> GSHHHHHHSIETDRVSKEFIEFLKTFHKTGQEIYKQTKLFLEGMHYKRDLSIEEQSECAQDFYHNVAERMQTRGKVPPERVEKIMDQIEKYIMTRLYKYVFCPETTDDEKKDLAIQKRIRALRWVTPQMLCVPVNEDIPEVSDMVVKAITDIIEMDSKRVPRDKLACITKCSKHIFNAIKITKNEPASADDFLPTLIYIVLKGNPPRLQSNIQYITRFCNPSRLMTGEDGYYFTNLCCAVAFIEKLDAQSLNLSQEDFDRYMSGQTSPRKQEAE;> GSRAYSFKVVLLGEGCVGKTSLVLRYCENKFNDKHITTLQASFLTKKLNIGGKRVNLAIWDTAGQERFHALGPIYYRDSNGAILVYDITDEDSFQKVKNWVKELRKMLGNEICLCIVGNKIDLEKERHVSIQEAESYAESVGAKHYHTSAKQNKGIEELFL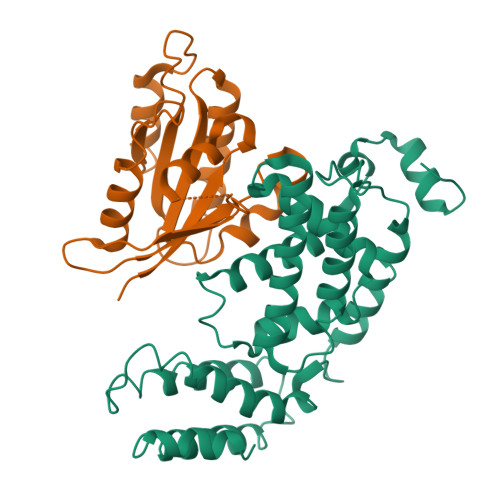DLCKRMIET> TVLPKDIPGDSLKVTVGTANGKPGDTVTVPVTFADVAKMKNVGTCNFYLGYDASLLEVVSVDAGPIVKNAAVNFSSSASNGTISFLFLDNTITDELITADGVFANIKFKLKSVTAKTTTPVTFKDGGAFGDGTMSKIASVTKTNGSVTIDP;> VIVYGDYNNDGNVDSTDFAGLKKYIMAADHAYVK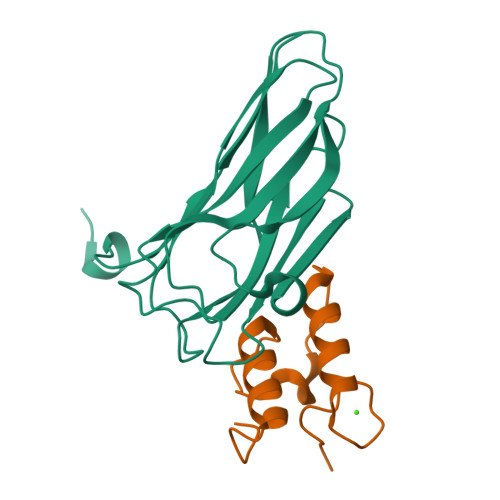NLDVNLDNEVNAFDLAILKKYLLGMVSKLE In this study, we identify a β-galactosidase with novel substrate specificity from Bacteroides xylanisolvens, an intestinal bacterium. The gene encoding the Bxy_22780 protein in the GH35 family is a component of a gene cluster containing SusC-like and SusD-like proteins. In this study, we found that Bxy_22780 specifically hydrolyzes β-1,2-galactooligosaccharides. We propose β-1,2-galactooligosaccharide galactohydrolase as a systematic name and β-1,2-galactosidase as an accepted name for Bxy_22780.

To learn more about the binding modes of the natural substrates determined above, the ligand-free enzyme structure of the E350G mutant and the complex structures of the WT enzyme with galactose and methyl β-galactopyranoside (MeβGal) were determined at resolutions of 1.91, 1.86, and 1.94 Å, respectively. In the WT-MeβGal complex, the electron density of MeβGal was clearly observed only at subsite +1. MeβGal is firmly recognized by Bxy_22780. In MeβGal, the 2- and 3-hydroxy groups form hydrogen bonds with Asn119 and Glu190, and its 3- and 4-hydroxy groups form water-mediated hydrogen bonds with the main chain atoms in Leu289, Gln291, Asp326, and Tyr328. The indole ring of Trp288 hydrophobically interacts with the six-membered ring in MeβGal. The 2-hydroxy group of MeβGal is oriented toward subsite −1 and is located close to an anomeric hydroxy group in the superimposed galactose molecule at subsite −1. Moreover, Glu190, a putative acid/base residue, interacts with the 2-hydroxy group of MeβGal. The methyl group in MeβGal faces the solvent, which is consistent with the result that Bxy_22780 acts on β-1,2-Gal3. Thus, the complex structure suggests that orientations of 2-, 3-, and 4-hydroxy groups and the orientation of the pyranose ring determine the substrate specificity of Bxy_22780.

>MRPPMYTSTNTEVPSRLVKNEHGSWQLIVNGKPFIMLAGELHNSSASTTEYLNSLWTSLKTLNLNTVLAPIAWEQFEPQEGIFDYTLINNMIDGARKNGFKLSILWFGSWKNGESSYAPTWVKEDTKRFFRVKSVEGKEIETISPFCENAMKADAKAFKTLVEHIKKVDQATGTVIALQPENEVGIFQGMDYSKASLAAYEQEVPQALIQYMKKNRKNLRKELLSVWEENGARTSGAWKTVFGDNAWSKSFYTTWQYATYIDFISAGAKEIYPLPTFCNCWLVQKPDDMPGVYPNGGPVSRVMDIWKAAAPHIDVLAPDIYLSDFKNIVADYHRADNPLLIPEAVMKPANAFWAFGEHSALCYSPFGIEDGADNFVFAQSYKVLNELIPLISEHQGSDRMIGVMKMPGESERTVTMGDYQLCIKYDAEDAYGLIIQTGKNEFVVAGINFKVYFTSTDKKKTGYIKQVWEGGYDTDGEWKATRLLNGDETYHNAVLIAKGRRTFTSEKSNNYNADHSDEIFVYSPTSYQAVWSPGIYRVTTYLRLEHHHHHH[4x]>SNILEMTKNYYDRSVSPVEYAYFDQSQNMRAINWNKIVDEKDLEVWNRVTQNFWLPENIPVSNDLPSWNELDDDWQQLITRTFTGLTLLDTVQSSIGDVAQIKNSLTEQEQVIYANFAFMVGVHARSYGTIFSTLCTSEQIEEAHEWVVDNEALQARPKALIPFYTADDPLKSKIAAALMPGFLLYGGFYLPFYLSARGKLPNTSDIIRLILRDKVIHNFYSGYKYQLKVAKLSPEKQAEMKQFVFDLLDKMIGLEKTYLHQLYDGFGLADEAIRFSLYNAGKFLQNLGYESPFTKEETRIAPEVFAQLSARADENHDFFSGSGSSYIIGTSEETLDEDWDF[4x];>SNILEMKELIVYFSTQSNNTHRFVQKLDAESIRIPIDEEERIKVDEDYV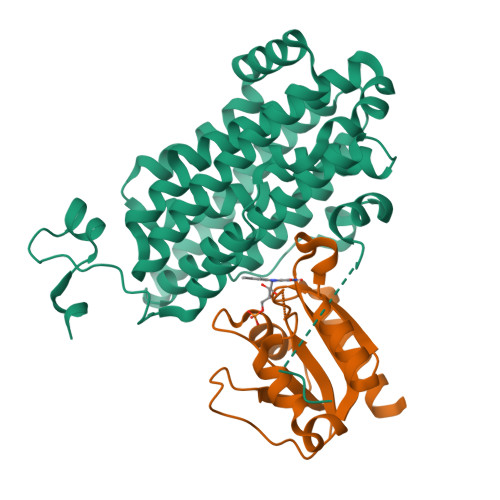LIVPTYSGGKVTDAGQVDAHGAVPKQVIHFLNDPDNRKHCLGVISSGNTNFGDSFAIAGPVISYKLKVPLLYQFELIGTKEDVEEVNRIISETFNADQ[4x]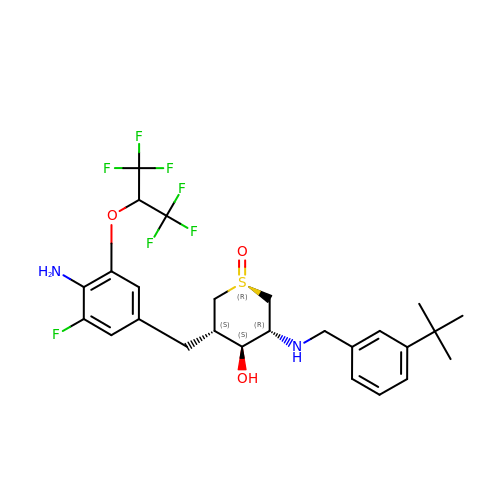(1R,3S,4S,5R)-3-{4-amino-3-fluoro-5-[(1,1,1,3,3,3-hexafluoropropan-2-yl)oxy]benzyl}-5-[(3-tert-butylbenzyl)amino]tetrahydro-2H-thiopyran-4-ol 1-oxide | C26 H31 F7 N2 O3 S | SVZBUJIOBQPGEC-UDLQCLCKSA-N>XGEVAQAIKEVAKAIKEVAWAIKEVAQA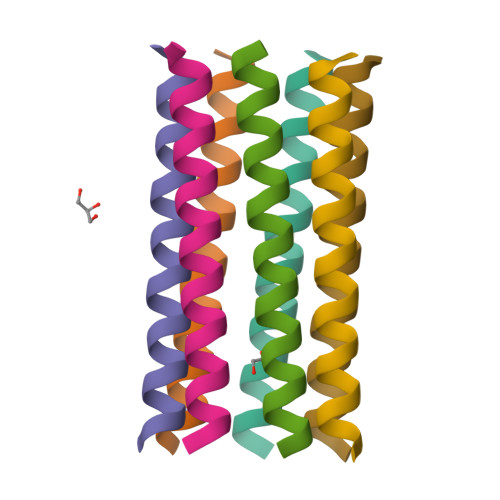IKGX[7x]>MFDRLKNGEKIAPIVKEVESQITEVHKRADEVIESNQFRVLESFGKHKISDSHFIPTTGYGYDDIGRDTLEKVYADVFGAEAGLVRPQIISGTHAISTALFGILRPGDELLYITGKPYDTLEEIVGVRGKGVGSFKEYNIGYNAVPLTEGGLVDFEAVAAAIHSNTKMIGIQRSKGYATRPSFTISQIKEMIAFVKEIKPDVVVFVDNCYGEFIEEQEPCHVGADLMAGSLIKNPGGGIVKTGGYIVGKEQYVEACAYRLTSPGIGAEAGASLYSLQEMYQGFFLAPHVAGQALKGAIFTAAFL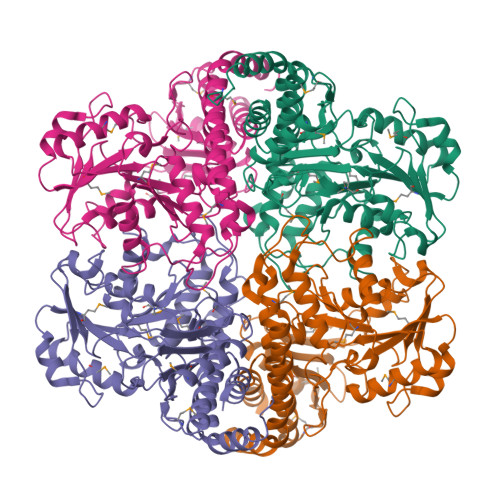EKLGMNTSPAWNAPRTDLIQSVQFDDKDRMIAFCQAIQYASPINSHFTPYANYMPGYEDDVIMAAGTFIQGASIELSADGPIRPPYVAYVQGGLTYSHVKIAICSAIDELIEKNLLTISLEHHHHHH[8x]> MSKPQPIAAANWKCNGSQQSLSELIDLFNSTSINHDVQCVVASTFVHLAMTKERLSHPKFVIAAQNAIAKSGAFTGEVSLPILKDFGVNWIVLGHSERRAYYGETNEIVADKVAAAVASGFMVIACIGETLQERESGRTAVVVLTQIAAIAKKLKKADWAKVV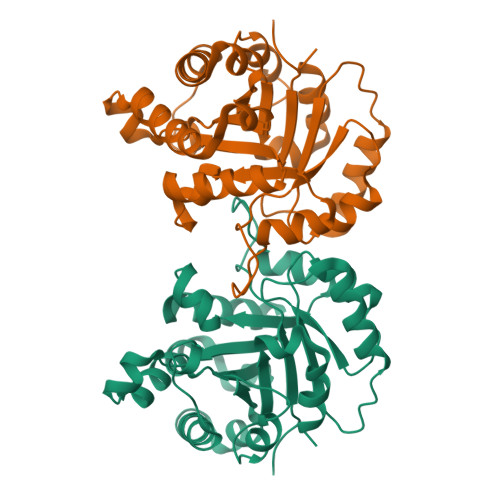IAYEPVWAIGTGKVATPQQAQEAHALIRSWVSSKIGADVRGELRILYGGSVNGKNARTLYQQRDVNGFLVGGASLKPEFVDIIKATQ> MSVVIDYNVAPPNLSTLPNGSLFETWRPRAHVLPPNGQIGDPCLHYTDPATGLFHVGFLHDGSGISSATTDDLATYQDLNQGNQVIVPGGINDPVAVFDGSVIPNGINGLPTLLYTSVSYLPIHWSIPYTRGSETQSLAVSSDGGSNFTKLDQGPVIPGPPF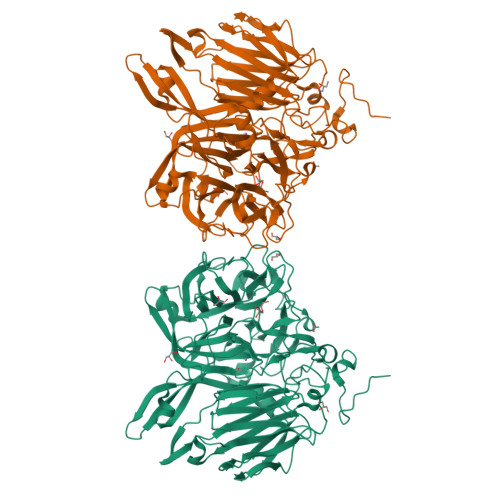AYNVTAFRDPYVFQNPTLDSLLHSKNNTWYTVISGGLHEKGPAQFLYRQYDSDFQYWEYLGQWWHEPTNSTWGNGTWAGRWAFNFETGNVFSLDEYGYNPHGQIFTTIGTEGSDLPVVPQLTSIHDMLWVSGTVSRNGSVSFNPNMAGFLDWGFSSYAAAGKVLPSTSLPSTKSGAPDRFISYVWLSGDLFEQAEGFPTNQQNWTGTLLLPRELRVLYIPNVVDNALARESGASWQVVSSDGSAGTVELQTLGISIARETKAALLSGTSFTESGRTLNSSGVVPFKRSPSEKFFVLSAQLSFPASARGSGLKSGFQILSSEHESTTVYYQFSNESIIVDRSNTSAAARTTDGIDSSAEAGKLRLFDVLNGGEQAIETLDLTLVVDNSVLEVYANGRFALSTWVRSWYANSTNISFFHNGVGGVAFSKVTVSEGLYDAWPDRQY>GGMTAFSTLNVLPPAQLTNLNELGYLTMTPVQAAALPAILAGKDVRVQAKTGSGKTAAFGLGLLQQIDASLFQTQALVLCPTRELADQVAGELRRLARFLPNTKILTLCGGQPFGMQRDSLQHAPHIIVATPGRLLDHLQKGTVSLDALNTLVMDEADRMLDMGFSDAIDDVIRFAPASRQTLLFSATWPEAIAAISGRVQRDPLAIEIDSTDALPPIEQQFYETSSKGKIPLLQRLLSLHQPSSCVVFCNTKKDCQAVCDALNEVGQSALSLHGDLEQRDRDQTLVRFANGSARVLVATDVAARGLDIKSLELVVNFELAWDPEVHVHRIGRTARAGNSGLAISFCAPEEAQRANIISDMLQIKLNWQTPPANSSIATLEAEMATLCIDGGKKAKMRPGDVLGALTGDIGLDGADIGKIAV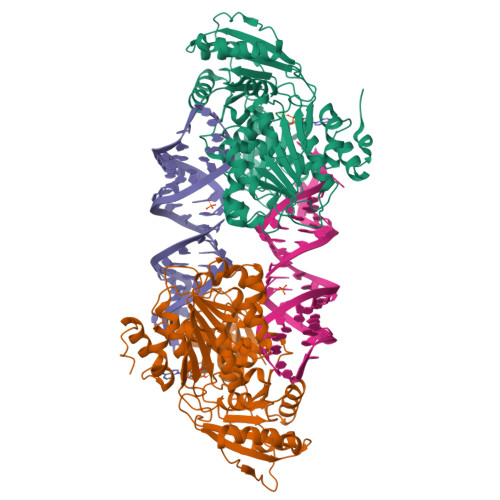HPAHVYVAVRQAVAHKAWKQLQGGKIKGKTCRVRLLK[4x]>PALVQRRKKVAMIGSGMIGGTMGYLCALRELADVVLYDVVKGMPEGKALDLSHVTSVVDTNVSVRAEYSYEAALTGADCVIVTAGLTKVPGKPDSEWSRNDLLPFNSKIIREIGQNIKKYCPKTFIIVVTNPLDCMVKVMCEASGVPTNMICGMACMLDSGRFR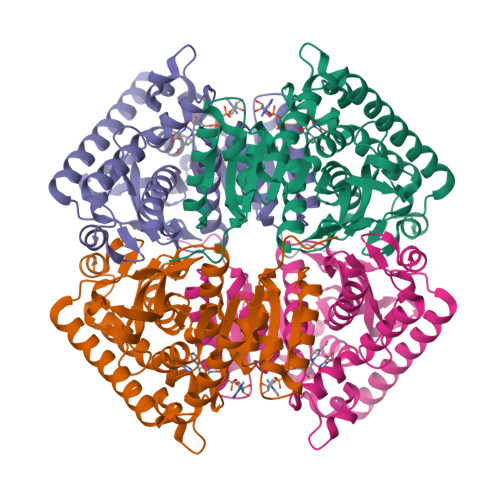RYVADALSVSPRDVQATVIGTHGDCMVPLVRYITVNGYPIQKFIKDGVVTEKQLEEIAEHTKVSGGEIVRFLGQGSAYYAPAASAVAMATSFLNDEKRVIPCSVYCNGEYGLKDMFIGLPAVIGGAGIERVIELELNEEEKKQFQKSVDDVMALNKAVAALQAPG[4x]> MLIKKALTAVALLASLLGASAAFAHAHLKSATPAADSTVAAPAD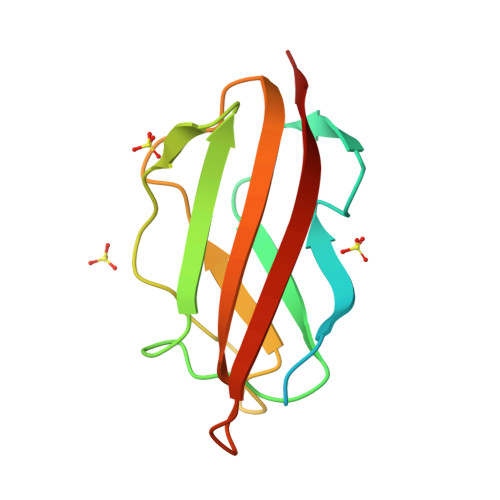LRLTFSEGVEATFTKVSLSKDGTEVAIKGLETPDADKKTLVVTPAAPLAAGNYKVVWNAVSVDTFKSNGEYSFKVKKK>MADSDPGERSYDNMLKM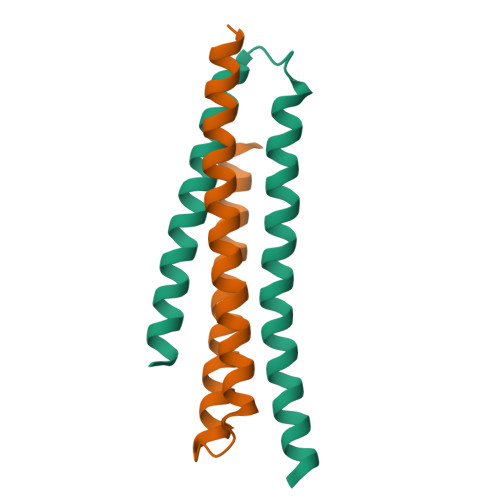LSDLNKDLEKLLEEMEKISVQATWMAYDMVVMRTNPTLAESMRRLEDAFLNCKEEMEKNWQELLTETKRKQ[2x]4-[(1R,2S)-1-ethyl-2-(4-hydroxyphenyl)butyl]phenol 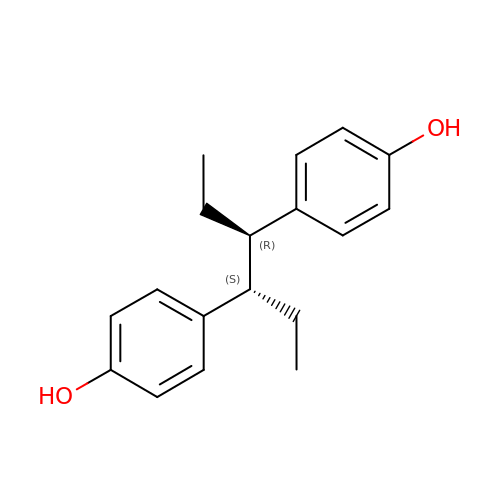| C18 H22 O2 | PBBGSZCBWVPOOL-HDICACEKSA-N In particular, the Hantaviridae family comprises the virus Hantaan (HTNV) that gives rise to haemorrhagic fevers with renal syndrome and the virus Sin Nombre that is linked to severe pulmonary illnesses with fatality rates up to 40%. The Bunyavirales genome is usually divided into three RNA segments enwrapped by the viral nucleoproteins (NP). The resulting nucleocapsids (NCs) protect the genome and serve as a replication/transcription template for the viral polymerase. In this context, HTNV-NCs are intriguing as they were shown to be able to form rather rigid helices of 10 nm diameter within viruses and during cell infection.

Expression of recombinant full-length HTNV-NP in insect cells led to formation of recombinant NCs that have a diameter consistent with native NCs. Cryo-EM images collected on a Titan Krios enabled structural determination of HTNV-NC at 3.3 Å resolution (Figure 1—figure supplements 1 and 2, Figure 1—source data 1). HTNV-NC is a left-handed helix with a pitch of 68.03 Å and 3.6 subunits per turn. The structure of NP80-429 is composed of a core comprising residues 117 to 398 (NPcore) that defines two lobes surrounding a positively charged groove. As a result, Nt- and Ctarm of the same subunit embrace each other: residues 97–98 of Ntarm contact residues 423–424 of Ctarm, revealing a unique intra-arms interaction specific to HTNV-NC. Successive subunit interactions rely on exchange of their Ntarm, and Ctarm that make intimate contacts with the core domain of neighbouring protomers, resulting in a buried area of 2704 Å2 at each NP-NP interface. The two β-strands of the hairpin (residues 155–160 and 177–181) interact with the Ntarm residues 101–103 from the following subunit to form a 3-stranded β-sheet. In addition, the β-hairpin152-181 tip (residues 162–175) acts as a clamp and seals the C-terminus-mediated contacts between NPi+2 (residues 409 to 419) and NPi+3 (residues 385–390), thereby buttressing and rigidifying the metastable helical form of the HTNV-NC. Consistently, three nucleotides with a partial occupancy can be visualised for each NP. Conserved residues R197, R314, R368, R146 and K153 interact via salt bridges with RNA phosphates, in line with the versatility of RNA sequence to be incorporated by NP. The nucleotides bind in a continuous positively charged groove oriented towards the interior of the NC.

> GMATMEELQREINAHEGQLVIARQKVRDAEKQYEKDPDELNKRTLTDREGVAVSIQAKIDELKRQLADRIATGKNLGKEQDPTGVEPGDHLKERSMLSYGNVLDLNHLDIDEPTGQTADWLSIIVYLTSFVVPILLKALYMLTTRGRQTTKDNKGTRIRFKDDSSFEDVNGIRKPKHLYVSLPNAQSSMKAEEITPGRYRTAVCGLYPAQIKARQMISPVMSVIGFLALAKDWSDRIEQWLIEPCKLLPDTAAVSLLGGPATNRDYLRQRQVALGNMETKESKAIRQHAEAAGCSMIEDIESPSSIWVFAGAPDRCPPTCLFIAGIAELGAFFSILQDMRNTIMASKTVGTSEEKLRKKSSFYQSYLRRTQSMGIQLGQRIIVLFMVAWGKEAVDNFHLGDDMDPELRTLAQSLIDVKVKEISNQEPLKL adenylyl-2"-tobramycin 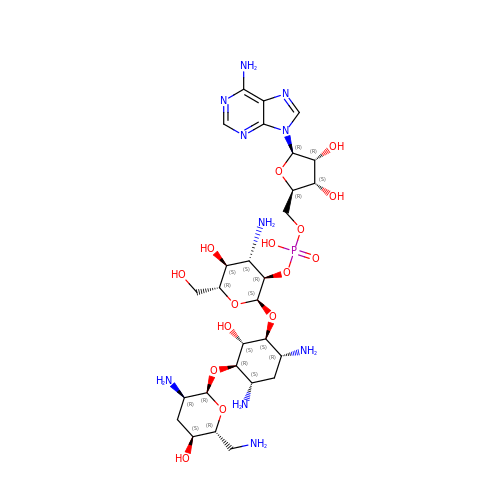| C28 H49 N10 O15 P | RHQLHNATZATWNZ-XMUWNKPOSA-N> GNVARVVVWEWLNEHSRWRPYTATVCHHIENVLKEDARGSVVLGQVDAQLVPYIIDLQSMHQFRQDTGTMRPVRRNFYDPSSAPGKGIVWEWENDGGAWTAYDMDICITIQNAYEKQHPWLDLSSLGFCYLIYFNSMSQMNRQTRRRRRLRRRLDLAYPLTVGSI

The WWE domain is a relatively under-researched domain found in twelve human proteins and characterized by a conserved tryptophan-tryptophan-glutamate (WWE) sequence motif. Six of these WWE domain-containing proteins also contain domains with E3 ubiquitin ligase activity. Here, we present novel crystal structures of the HUWE1, TRIP12, and DTX1 WWE domains in complex with PAR building blocks and their analogs, thus enabling a comprehensive analysis of the PAR binding site structural diversity. A highly conserved feature in all determined structures is the recognition and therefore the interactions involving the adenine ring of the ligands.

We solved two crystal structures of DTX1 in complex with ADP, with each structure having one ADP molecule bound to either of the two WWE domains. Our efforts to obtain a DTX1 co-crystal structure with both WWE domains bound to ADP were unsuccessful despite having excess ADP in our crystallization setups. To gain insight into why ADP ligands were only observed in one WWE domain in our DTX1-ADP structures, we investigated conformational differences by comparing the bound and unbound WWE domains in the same structure. While the core structural elements appear to be conserved, some loop shifts are observed in both structures, with most differences occurring when ADP is bound to the WWE2 domain as compared to the unbound WWE1 domain in the DTX1-WWE2-ADP structure. The observed differences are in the loops that interact with the phosphate groups and may reduce the surface area of the ligand-binding site in the unbound WWE1 domain of the DTX1-WWE2-ADP structure, which therefore might discourage binding in the second site. Comparing our DTX1-WWE1-ADP and DTX1-WWE2-ADP co-crystal structures with the RNF146-iso-ADPr structure revealed that the residues at the corresponding distal ribose-phosphate moeities binding sites in DTX1 WWE domains may not support high affinity binding to iso-ADPr. Specifically, neither Trp30 nor Trp111 would allow for a direct hydrogen bond to the distal ribose oxygen, while residues in the loop regions (30–38 in WWE1 and 111–122 in WWE2) would not contribute to high affinity binding to the distal phosphate group. Our biophysical data, however, supports DTX1 preference for iso-ADPr over ADPr, which may indicate a mechanism where it recognizes PAR via both iso-ADPr and ADP moieties.> CETAPKEVVYVEGAVEASLTGAPGNPEE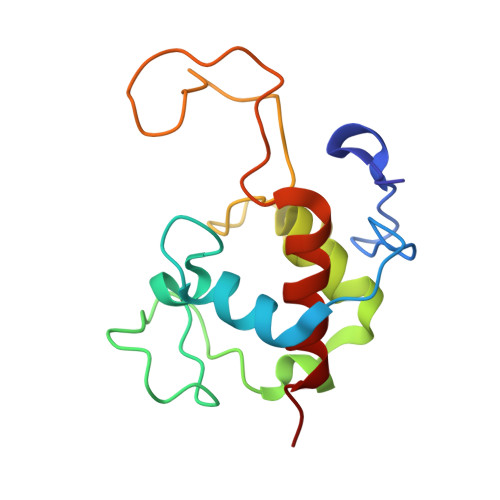GVRIMTTNALGNCVACHQIGALPDVEFPGTIAPPLDGAGDRWTEAQLRGIVANAKMTFEGTFMPAFYKVDGFVRPGDGFSGKAGAEPLAPILNAQQIEDVVAFLVTLKE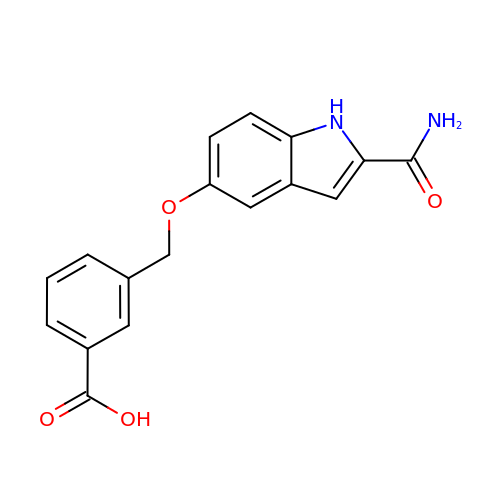3-[(2-aminocarbonyl-1~{H}-indol-5-yl)oxymethyl]benzoic acid | C17 H14 N2 O4 | JPBFPBAFCGZOAS-UHFFFAOYSA-N>MA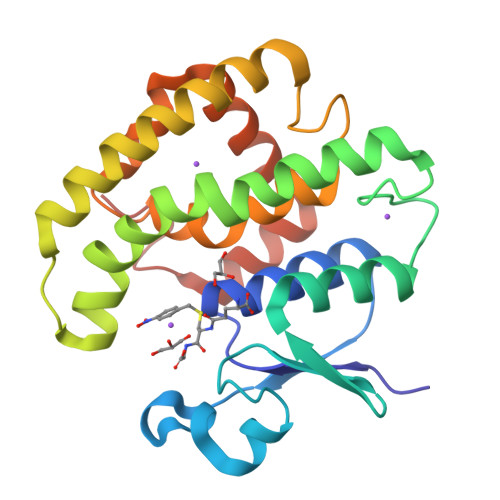PVKVFGPAMSTNVARVLVFLEEVGADYEVVDMDFKVMEHKSPEHLARNPFGQIPAFQDGDLLLFESRAISKYVLRKYKTGEVDLLREGNLKEAAMVDVWTEVDAHTYNPALSPIVYQCLFNPMMRGIPTDEKVVAESLEKLKKVLEVYEARLSQHEYLAGDFVSFADLNHFPYTFYFMATPHAALFGSYPHVKAWWERIMARPAIKKISATMVPPKAKGHHHHHH[6x]>GGCGCUUGCGUC[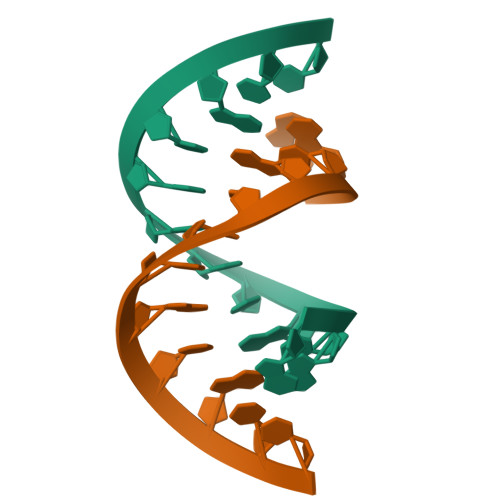4x]> MYDASLIPNLQIPQKNIPNNDGMNFVKGLRLGWNLGNTFDAFNGTNITNELDYETSWSGIKTTKQMIDAIKQKGFNTVRIPVSWHPHVSGSDYKISDVWMNRVQEVVNYCIDNKMYVILNTHHDVDKVKGYFPSSQYMASSKKYITSVWAQIAARFANYDEHLIFEGMNEPRLVGHANEWWPELTNSDVVDSINCINQLNQDFVNTVRATGGKNASRYLMCPGYVASPDGATNDYFRMPNDISGNNN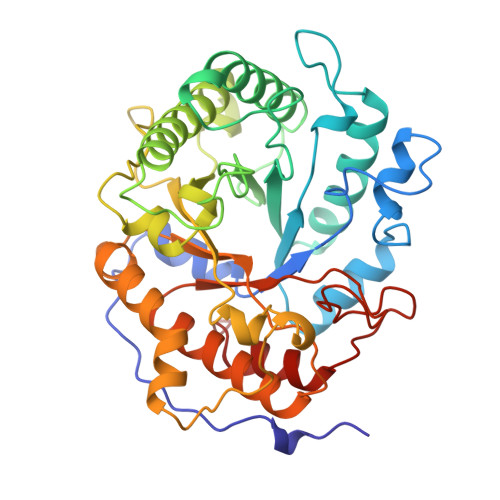KIIVSVHAYCPWNFAGLAMADGGTNAWNINDSKDQSEVTWFMDNIYNKYTSRGIPVIIGECGAVDKNNLKTRVEYMSYYVAQAKARGILCILWDNNNFSGTGELFGFFDRRSCQFKFPEIIDGMVKYAFGLIN> STWGSLKTSAVPSTSTMSQEPELL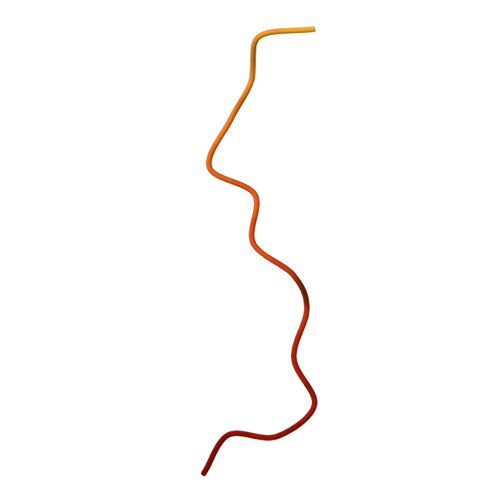ISGMEKPLPLRTDFS> SYTHLSFYEKRELFRKKLREIEGPEVTLVNEVDDEPCPSLDFQFISQYRLTQGVIPPDPNAQSGCNCSSLGGCDL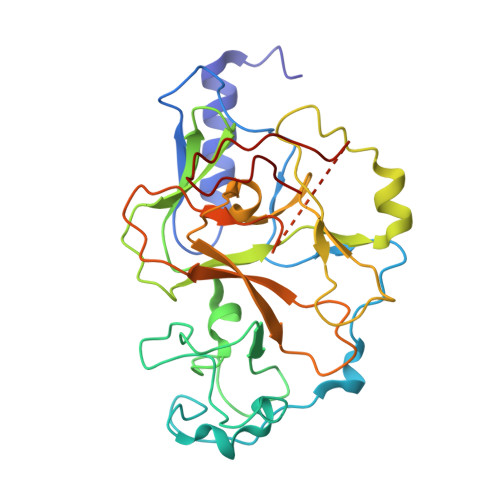NNPSRCECLDDLDEPTHFAYDAQGRVRADTGAVIYECNSACSCSMECPNRVVQRGRTLPLEIFKTKEKGWGVRSLRFAPAGTFITCYLGEVITSAEAAKRDKNYDDDGITYLFDLDMFDDASEYTVDAQNYGDVSRFFNHSCSPNIAIYSAVRNHGARTIYDLAFFAIKDIQPLEELTFDYAGAKDFSPVQSQKSQQNRISKLRRQCKCGSANCRGWLF>[2x]MESCYNPGLDGIIEYDDFKLN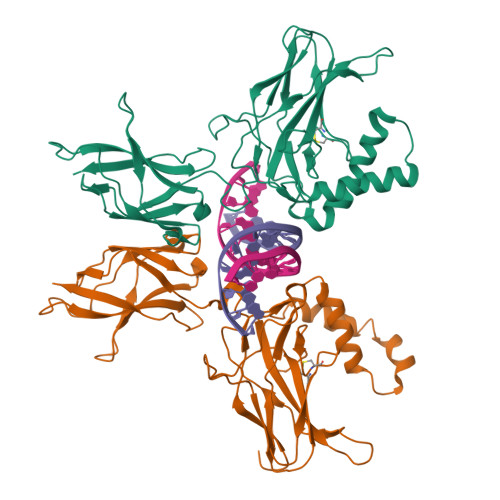SSIVEPKEPAPETADGPYLVIVEQPKQRGFRFRYGCEGPSHGGLPGASSEKGRKTYPTVKICNYEGPAKIEVDLVTHSDPPRAHAHSLVGKQCSELGICAVSVGPKDMTAQFNNLGVLHVTKKNMMGTMIQKLQRQRLRSRPQGLTEAEQRELEQEAKELKKVMDLSIVRLRFSAFLRASDGSFSLPLKPVISQPIHDSKSPGASNLKISRMDKTAGSVRGGDEVYLLCDKVQKDDIEVRFYEDDENGWQAFGDFSPTDVHKQYAIVFRTPPYHKMKIERPVTVFLQLKRKRGGDVSDSKQFTYYP The HAdV-D36 fiber knob domain (FK), which mediates the primary attachment of many HAdVs to host cells, has a significantly elongated DG loop that alters known binding interfaces for established adenovirus receptors such as the coxsackie- and adenovirus receptor (CAR) and CD46. Our data suggest that HAdV-D36 attaches to host cells using a versatile receptor pool comprising sialic acid-containing glycans and CAR. Sialic acids are recognized at the same binding site used by other HAdVs of species D such as HAdV-D37. Using glycan microarrays, we demonstrate that HAdV-D36 displays a binding preference for glycans containing a rare sialic acid variant, 4-O,5-N-diacetylneuraminic acid, over the more common 5-N-acetylneuraminic acid.

In contrast, 4-O-acetylated Neu5Ac is expressed in fewer species and has so far not been detected in humans. N313 is one of the residues of the conserved VSN stretch and closes the binding pocket from below. Interestingly, the O-acetyl function does not contribute any polar contact and instead induces the tilting movement under the steric influence of the bulky side chains of Y315 and P323. This interaction is supposedly not favorable for the binding; however, the steric constraints bring the O-acetyl groups of the three sugar moieties into a position in which they contact each other by means of a triangular hydrophobic interaction (mean distance between methyl C atoms: 4.3 Å) that displaces water molecules in the area. A similar effect is not expected for Neu5Ac. Interestingly, all known complex structures with 4,5-acetylated SA display a similar arrangement.

>[3x]MSKRLRVEDDFNPVYPYGYARNQNIPFLTPPFVSSDGFQNFPPGVLSLKLADPIAIANGNVSLKVGGGLTVEQQSGKLSVDTKAPLQVANDNKLELSYDDPFKVENNKLGIKAGHGLAVVTKENTSLPSLVGTLVVLTGKGIGTGSSAHGGTIDVRLGEGGGLSFDEKGDLVAWDKKNDTRTLWTTPDPSPNCKVETARDSKLTLALTKCGSQILATVSLLVVTGKYAIISDTVNPKQFSIKLLFNDKGVLLSDSNLDGTYWNYRSNNNNIGTPYKEAVGFMPSTTAYPKPTNNTSTDPDKKVSQGKNKIVSNIYLGGEVYQPGFIVVKFNQETDANCAYSITFDFGWGKVYKDPIPYDTSSFTFSYIAQE>MSFFHGVTVTNVDIGARTIALPASSVIGLCDVFTPGAQASAKPNVPVLLTSKKDAAAAFGIGSSIYLACEAIYNRAQAVIVAVGVETAETPEAQASAVIGGISAAGERTGLQALLDGKSRFNAQPRLLVAPGHSAQQAVATAMDGLAEKLRAIAILDGPNSTDEAAVAYAKNFGSKRLFMVDPGVQVWDSATNAARNAPASAYAAGLFAWTDAEYGFWSSPSNKEIKGVTGTSRPVEFLDGDETCRANLLNNANIATIIRDDGYRLWGNRTLSSDSKWAFVTRVRTMDLVMDAILAGHKWAVDRGITKTYVKDVTEGLRAFMRDLKNQGAVINFEVYADPDLNSASQLAQGKVYWNIRFTDVPPAENPNFRVEVTDQWLTEVLDVA[24x];>MMIPQTLTNTNLFIDGVSFAGDVPSLTLPKLAVKTEQYRAGGMDAPVSIDMGLEAMEAKFSTNGARREALNFFGLADQSAFNGVFRGSFKGQKGASVPVVATLRGLLKEVDPGDWKAGEKAEFKYAVAVSYYKLEVDGREVYEIDPVNGVRAINGVDQLAGMRNDL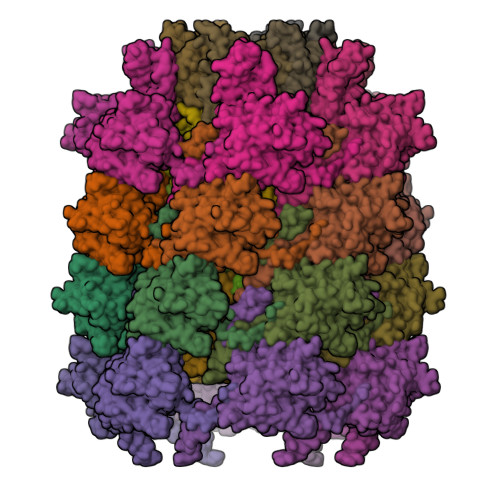GL[24x]13-ACETYLPHORBOL | C22 H30 O7 | 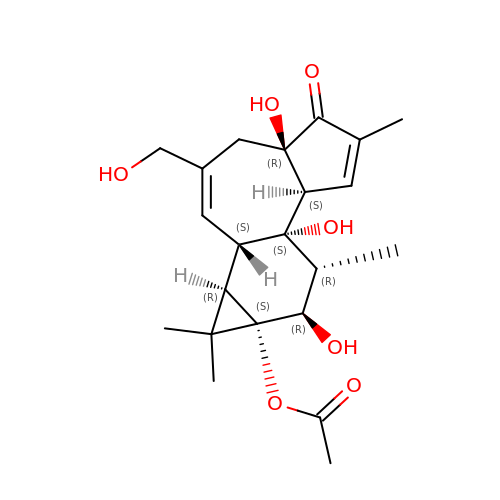SDSVJYOOAPRSDA-RPCQODIISA-N>ACLNTRFLEEEELRSHHILERLDAHI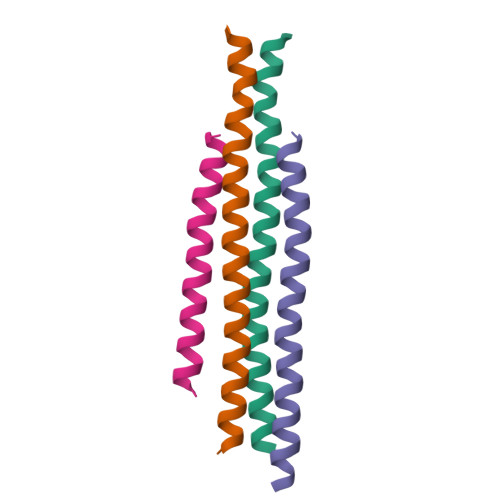EELKRESEKTVRQFTALK[2x];>[2x]MGALEELRGQYIKAVKKIKCDMLRYIQESKERAAEMVKAEVLRERQETARKMRK>SENVSLNNISMQILRELLQYRRHLTDPVKNSAKEEEIIKTVQLPRIEYFIKNKKPIEFILPAFPTKSPNINKVLGTAPDMAERLSLIFLNSFCQRIQLYYPPGARIIICSDGHVFGDLIHVSDEVISQYHEDIKQLLHEVGAINLSTFNLNDDKELAEHSDDFNLQRQMLVKHYARSEASIKDELLQNNNGLQLYRAVTRFLYEDSLLPGYTGSNNALQKDAKQRAIGVIQRSWAWGSLLDTHFPKAIRLSIHPQPADSIKFGIHMMPTRDDWLTPWH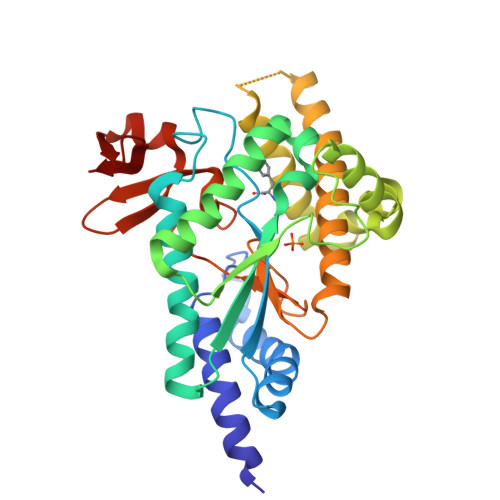GVAANVNGQFILMKHKEVQMMGGKLVNIHGKPSHYVI[2x]C2-HYDROPEROXY-COELENTERAZINE | C26 H21 N3 O5 | 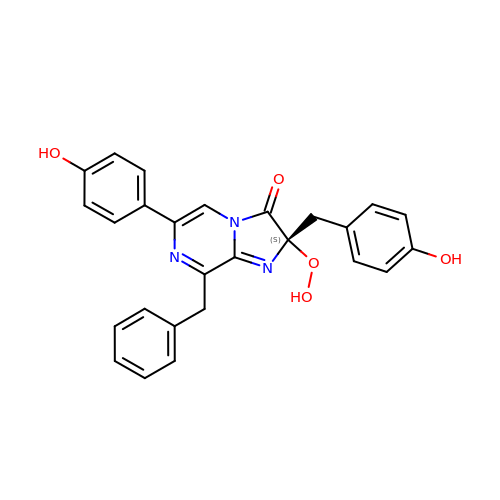HOSWCJDTHOAORT-SANMLTNESA-N>[3x]MKRKPNSNQNNNNNRGNGNGLRRVRGGRVSRRRVVINQSNQSMPVTSNGAPLQALTSYSRPNVNKISRLGPDSDFLTSVVAKASTSIVTPADRILVKQPLSASSFPGTRITGLSSYWE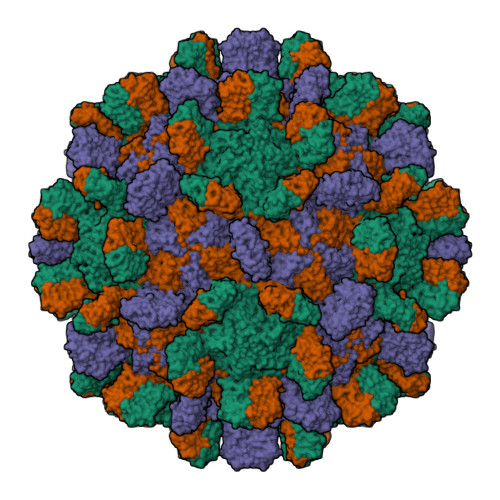RYKWLSAVARYVPAVPNTVACQFVMYIDTDPLDDPSNISDDNQIVRQAVSQAGSNQFNFNTSKTVPLIVRADNQYYYTGVDKQNLRFSLQGILYIIQVTDLINFNGELITQDLTCGSLFLDWLVNFSIPQINPTSLTDVRVDKAVNFIKPEVSGVAEIQTVTGLSPSTSYLLTPAFLEQNFQSEAGIYILSATPVEGEGTISINMDPTVTTVSGFIKVKTDTFGTFDLSVVLTTASKKQTTGFNIIAATS>[4x]TIFQFPQDFMWGTATAAYQIEGAYQ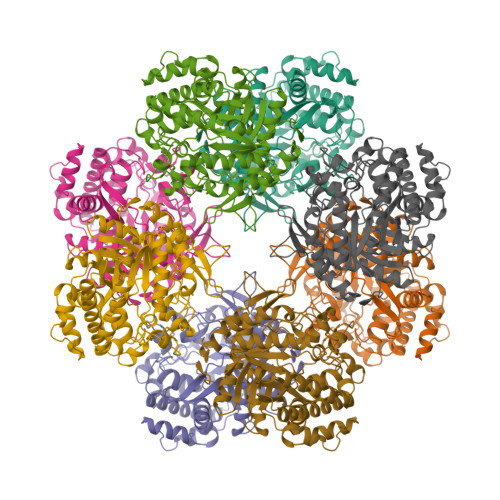EDGRGLSIWDTFAHTPGKVFNGDNGNVACDSYHRYEEDIRLMKELGIRTYRFSVSWPRIFPNGDGEVNQEGLDYYHRVVDLLNDNGIEPFCTLYHWDLPQALQDAGGWGNRRTIQAFVQFAETMFREFHGKIQHWLTFNEPWCIAFLSNMLGVHAPGLTNLQTAIDVGHHLLVAHGLSVRRFRELGTSGQIGIAPNVSWAVPYSTSEEDKAACARTISLHSDWFLQPIYQGSYPQFLVDWFAEQGATVPIQDGDMDIIGEPIDMIGINYYSMSVNRFNPEAGFLQSEEINMGLPVTDIGWPVESRGLYEVLHYLQKYGNIDIYITENGACINDEVVNGKVQDDRRISYMQQHLVQVHRTIHDGLHVKGYMAWSLLDNFEWAEGYNMRFGMIHVDFRTQVRTPKESYYWYRNVVSNNWLETRR> MSEMTPREIVSELDQHIIGQADAKRAVAIALRNRWRRMQLQEPLRHEVTPKNILMIGPTGVGKTEIARRLAKLANAPFIKVEATKFTEVGYVGKEVDSIIRDLTDSAMKLVRQQEIAKNRARAEDVAEERILDALLPPAKNQWGEVENHDSHSSTRQAFRKKLREGQLDDKEIEIDVSAGVSMGVEIMAPPGMEEMTNQLQSLFQNLGSDKTKKRKMKIKDALKALIDDEAAKLINPEELKQKAIDAVEQNGIVFIDEIDKICKKGEYSGADVSREGVQRDLLPLVEGSTVSTKHGMVKTDHILFIASGAFQVARPSDLIPELQGRLPIRVELTALSAADFERILTEPHASLTEQYKALMATEGVNIAFTTDAVKKIAEAAFRVNEKTENIGARRLHTVMERLMDKIS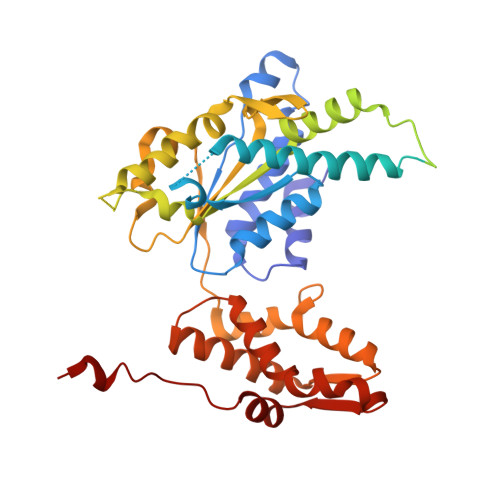FSASDMNGQTVNIDAAYVADALGEVVENEDLSRFIL>MDRPAVSGPMDLPIMHDSDRYELVKDIGSGNFGVARLMRDKQSNELVAVKYIERGEKIAANVK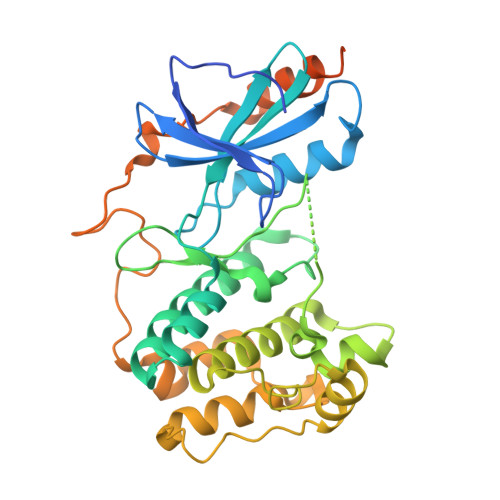REIINHRSLRHPNIVRFKEVILTPTHLAIVMEYASGGELFERICNAGRFSEDEARFFFQQLISGVSYCHAMQVCHRDLKLENTLLDGSPAPRLKICDFGYSKSSVLHSQPKSTVGTPAYIAPEVLLKKEYDGKVADVWSCGVTLYVMLVGAYPFEDPEEPKNFRKTIHRILNVQYAIPDYVHISPECRHLISRIFVADPAKRISIPEIRNHEWFLKNLPADLMNDNTMTTQFDESDQPGQSIEEIMQIIAEATVPPAGTQNLNHYLTGSLDIDDDMEEDLESDLDDLDIDSSGEIVYAM[2x]>[4x]MDLNLQDKVVIVTGGASGIGGAISMRLAEERAIPVVFARHAPDGAFLDALAQRQPRATYLPVELQDDAQCRDAVAQTIATFGRLDGLVNNAGVNDGIGLDAGRDAFVASLERNLIHYYAMAHYCVPHLKATRGAIVNISSKTAVTGQGNTSGYCASKGAQLALTREWAVALREH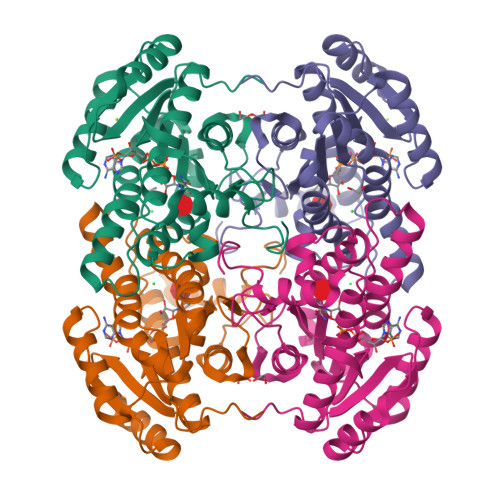GVRVNAVIPAEVMTPLYRNWIATFEDPEAKLAEIAAKVPLGRRFTTPDEIADTAVFLLSPRASHTTGEWLFVDGGYTHLDRALV> MPIRQMKDSSETHLVIKTQPLKHHNPKTVQNGKIPPPSPSPVTVTTPATVTQSQASSPSPPSKNRSRRRNRGGRKSDQGDVCMRPSSRPRKPPPPSQTTSSAVSVATAGEIVAVNHQMQMGVRKNSNFAPRPGFGTLGTKCIVKANHFLADLPTKDLNQYDVTITPEVSSKSVNRAIIAELVRLYKESDLGRRLPAYDGRKSLYTAGELPFTWKEFSVKIVDEDDGIINGPKRERSYKVAIKFVARANMHHLGEFLAGKRADCPQEAVQILDIVLRELSVKRFCPVGRSFFSPDIKTPQRLGEGLESWCGFYQSIRPTQMGLSLNIDMASAAFIEPLPVIEFVAQLLGKDVLSKPLSDSDRVKIKKGLRGVKVEVTHRANVRRKYRVAGLTTQPTRELMFPVDENCTMKSVIEYFQEMYGFTIQHTHLPCLQVGNQKKASYLPMEACKIVEGQRYTKRLNEKQITALLKVTCQRPRDRENDILRTVQHNAYDQDPYAKEFGMNISEKLASVEARILPAPWLKYHENGKEKDCLPQVGQWNMMNKKMINGMTVSRWACVNFSRSVQENVARGFCNELGQMCEVSGMEFNPEPVIPIYSARPDQVEKALKHVYHTSMNKTKGKELELLLAILPDNNGSLYGDLKRICETELGLISQCCLTKHVFKISKQYLANVSLKINVKMGGRNTVLVDAISCRIPLVSDIPTIIFGADVTHPENGEESSPSIAAVVASQDWPEVTKYAGLVCAQAHRQELIQDLYKTWQDPVRGTVSGGMIRDLLISFRKATGQKPLRIIFYRAGVSEGQFYQVLLYELDAIRKACASLEPNYQPPVTFIVVQKRHHTRLFANNHRDKNSTDRSGNILPGTVVDTKICHPTEFDFYLCSHAGIQGTSRPAHYHVLWDENNFTADGIQSLTNNLCYTYARCTRSVSIVPPAYYAHLAAFRARFYLEPEIMQDNGSPGKKNTKTTTVGD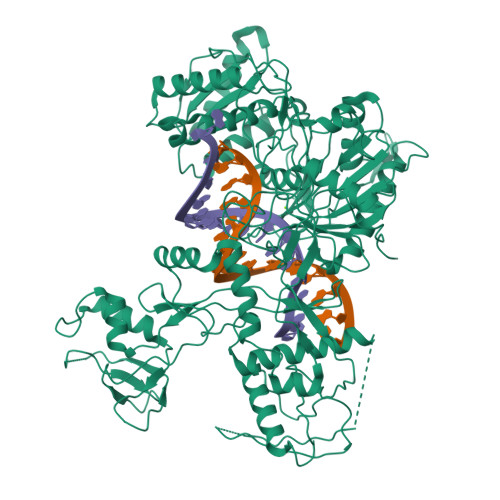VGVKPLPALKENVKRVMFYC> TRFTEEYQLFEELGKGAFSVVRRCVKVLAGQEYAAKIINTKKLSARDHQKLEREARICRLLKHPNIVRLHDSISEEGHHY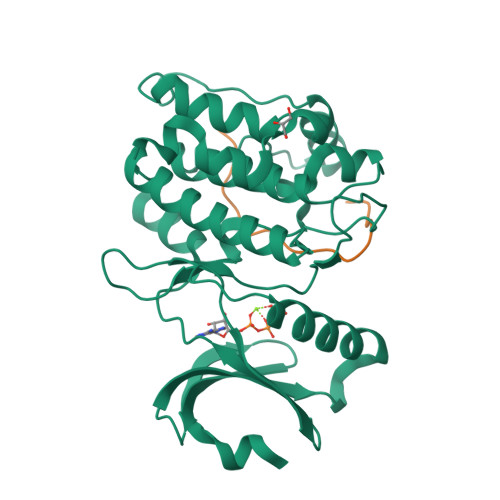LIFDLVTGGELFEDIVAREYYSEADASHCIQQILEAVLHCHQMGVVHRNLKPENLLLASKLKGAAVKLADFGLAIEVEGEQQAWFGFAGTPGYLSPEVLRKDPYGKPVDLWACGVILYILLVGYPPFWDEDQHRLYKQIKAGAYDFPSPEWDTVTPEAKDLINKMLTINPSKRITAAEALKHPWISHR;> KAQKKNRNKLRRQHDYDTFVDL> REFTIDFSTQQSYVSSLNSIRTEISTPLEHISQGTTSVSVINHTPPGSYFAVDIRGLDVYQARFDHLRLIIEQNNLAVAGFVNTATNTFYRFSDFTHISVPGVTTVSMTTDSSYTTLQRVAALERSGMQISRHSLVSSYLALMEFSGNTMTRDA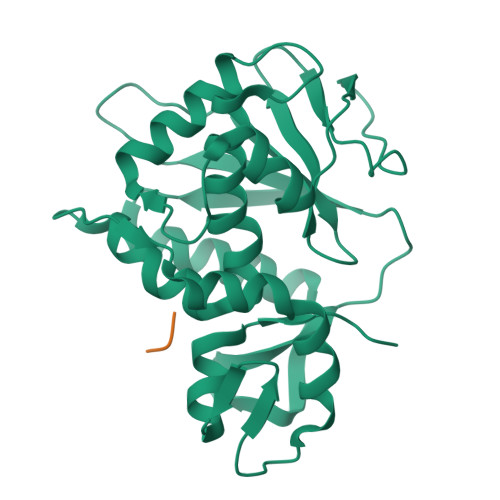SRAVLRFVTVTAEALRFRQIQREFRQALSETAPVYTMTPGDVDLTLNWGRISNVLPEYRGEDGVRVGRISFNNISAILGTVAVILNCHHQGARSVR;> GFGLFD3-methyl-L-valyl-L-prolyl-L-isoleucine | C17 H31 N3 O4 | 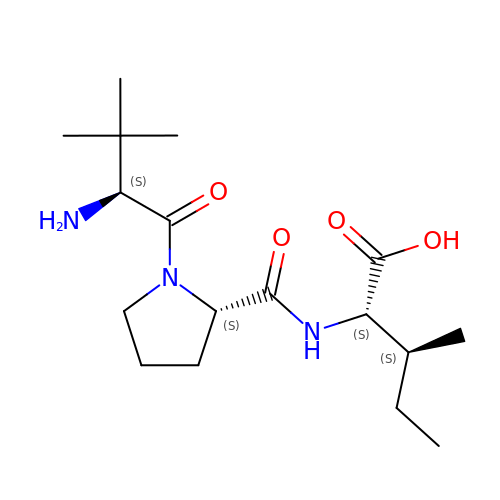SQVUEHPVMOLXQG-ZDEQEGDKSA-N>MKIVAIGAIPFSIPYTKPLRFASGEVHAAEHVLVRVHTDDGIVGVAEAPPRPFTYGETQTGIVAVIEQYFAPALIGLTLTEREVAHTRMARTVGNPTAKAAIDMAMWDALGQSLRLSVSEMLGGYTDRMRVSHMLGFDDPVKMVAEAERIRETYGINTFKVKVGRRPVQLDTAVVRALRERFGDAIELYVDGNRGWSAAESLRAMRE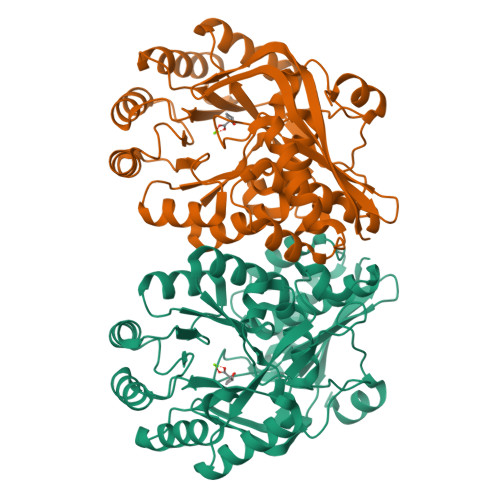MADLDLLFAEELCPADDVLSRRRLVGQLDMPFIADESVPTPADVTREVLGGSATAISIKTARTGFTGSTRVHHLAEGLGLDMVMGNQIDGQIGTACTVSFGTAFERTSRHAGELSNFLDMSDDLLTVPLQISDGQLHRRPGPGLGIEIDPDKLAHYRTDN[4x]>[3x]MAKKEKKRLQVVISEEQDALLTRAAYALSSPERAVSK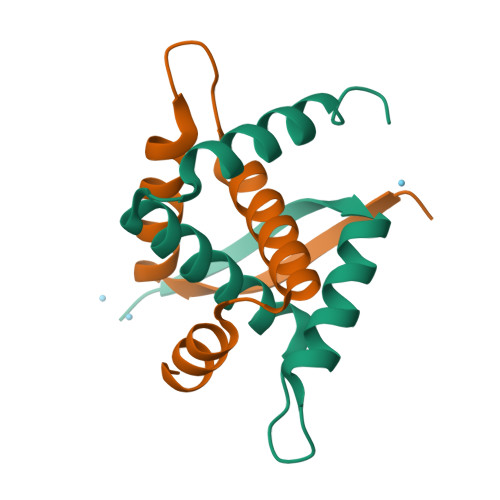SEVVRLAIEKIARELEEGKAKEELEALLKHLKAEEGEEEA>MMTTIAFLGLGNMGAPMSANLVGAGHVVRGFDPAPTAASGAAAHGVAVFRSAPEAVAEADVVITMLPTGEVVRRCYTDVLAAARPATLFIDSSTISVTDAREVHALAESHGMLQLDAPVSGGVKGAAAATLAFMVGGDESTLRRARPVLEPMAGKIIHCGAAGAGQAAKVCNNMVLAVQQIAIAEAFVLAEKLGLSAQSLFDVITGATGNC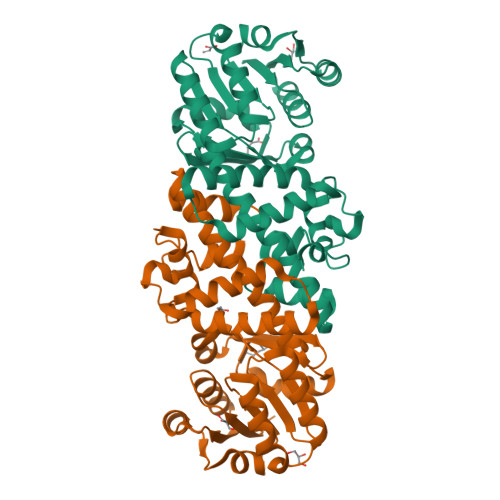WAVHTNCPVPGPVPTSPANNDFKPGFSTALMNKDLGLAMDAVAATGATAPLGSHAADIYAKFAADHADLDFSAVIHTLRARADA[2x]> MVKKNDLFVDVSSHNGYDITGILEQMGTTNTIIKISESTTYLNPCLSAQVEQSNPIGFYHFARFGGDVAEAEREAQFFLDNVPMQVKYLVLDYEDDPSGDAQANTNACLRFMQMIADAGYKPIYYSYKPFTHDNVDYQQILAQFPNSLWIAGYGLNDGTANFEYFPSMDGIRWWQYSSNPFDKNIVLLDDEEDDKPKTAGTWKQDSKGWWFRRNNGSFPYNKWEKIGGVWYYFDSKGYCLTSEWLKDNEKWYYLKDNGAMATGWVLVGSEWYYMDDSGAMVTGWVKYKNNWYYMT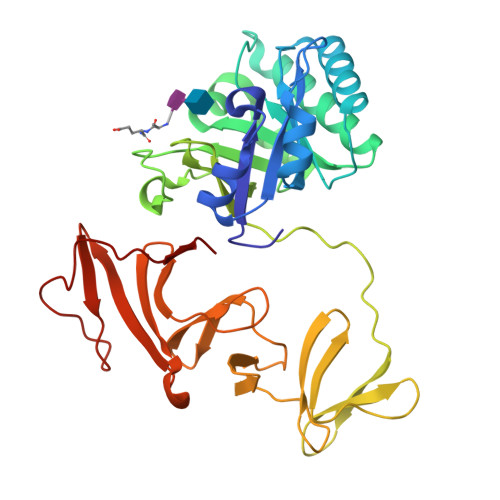NERGNMVSNEFIKSGKGWYFMNTNGELADNPSFTKEPDGLITVA> MNDMGSSEVNDENKEKEARYSVMTKSELEALAVSAIREHRRLLWADQAVYEEW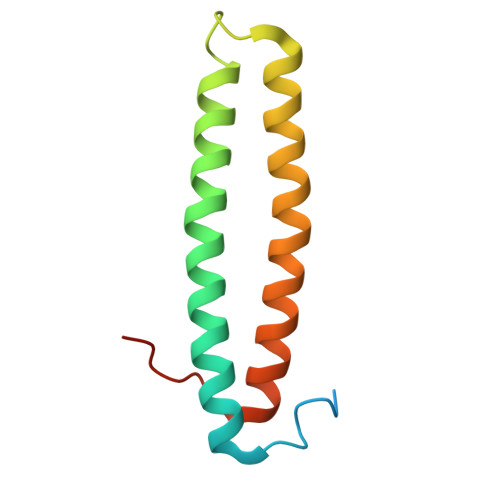LRASDDPSISGPVLQTLQDEYVARQKRSEAQQEELSDILDALGFVPDVPFDDDN5-(4-fluorophenyl)-2,3-dihydroxy-N-[(E)-5-pyrrolo[3,2-c]pyridin-1-ylpent-3-enyl]benzamide | C25 H22 F N3 O3 | 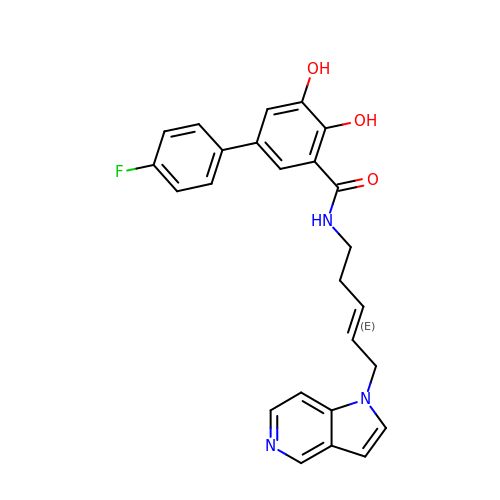MYCHLIVPJDYHPD-HNQUOIGGSA-N>[2x]MGKVIPKQEGLDHSVDFLREGYLFVANRRKSFQSNIFESRLLGERVICLGGEEAAEVFYDANKFTRQDAAPKRLLKTLFGEGGVQTLDGSEHTHRKQMFMSLMTKENIDRLLRLTYREWNQIERM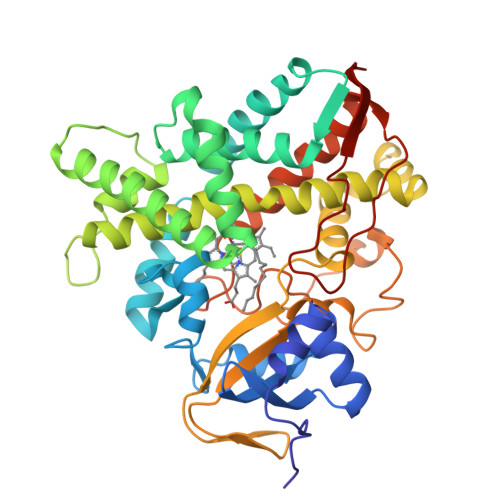GEEIVLYDIAQEVLMKAVCEWSGVPLAKEEVGKRTEEMRLLFESGTSLGPTYLQGRKARSSAEVWIRQMVKEVRSNRLLPNEHTALYEFSWHRDESGELLPEEVVAVEVLNILRPTVAISVYVLFTVLALHQFPDVKEQVERGEVSKTEFVQEVRRFYPFFPVAAARVKTDFEWDGYAFPEGTLTLLDLYGTNHDVSIWTEPDRFDPSRFKDWKESPFNFIPQGGGDVDFGHRCAGEHVTIAILAQVIELFTKEYAYTVPPQDLSYSFVDMPSLPKSKLRLTHLTRNQ>GSMASHGNAPPAPVGGAAQTHTQPPVQTAMRIALWNRATHGEQGALQHLLAGLWIQTEISPNSGDIHPLLFFDREHAEITFSRASVQEIFLVDSAHTHRKTVSFLTRNTA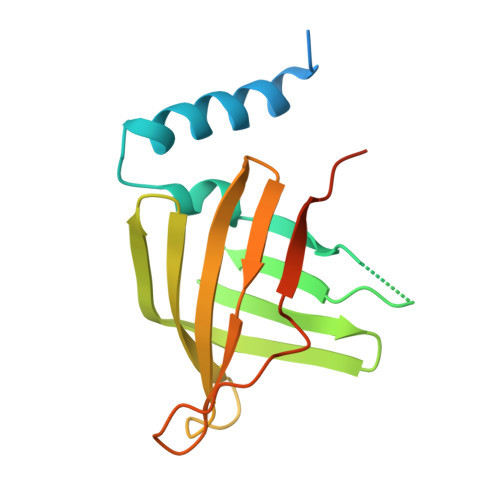ISSIRRRLEVTFESHAVIHVRAVEDVARLKIGSTSMWDGQYTRYHAGPASAPSPAAA[9x]>[2x]GTSTQTKAGSLTIVGTGIESIGQMTLQALSYIEAAAKVFYCVIDPATEAFILTKNKNCVDLYQYYDNGKSALNTYTQMSELMVREVRKGLDVVGVFYGHPGVFVNPSHRALAIAKSEGYRARMLPGVSAEDCLFADLCIDPSNPGCLTYEASDFLIRDRPVSIHSHLVLFQVGCVGIADFNFTGFDNNKFGVLVDRLEQEYGAEHPVVHYIAAMMPHQDPVTDKYTVAQLREPEIAKRVGGVSTFYIPPKARKASNLDIIRRLELLPAGQVPDKKARIYPANQWEPDVPEVEPYRPSDQAAIAQLADHAPPEQYQPLATSKAMSDVMTKLALDPKALADYKADHRAFAQSVPDLTPQERAALELGDSWAIRCAMKNMPSSLLDAARESGEEASQNGFPWVIVVGVIGVIG

While chemical methylation of an amide bond uses a strong base to generate the imidate, OphA, the precursor protein of the fungal peptide macrocycle omphalotin A, self-hypermethylates amides at pH 7 using S-adenosyl methionine (SAM) as cofactor. Omphalotin A derives from the C terminus of the OphA protein, and it is the OphA protein that methylates its own C terminus using S-adenosyl methionine (SAM). The structure of OphA reveals a complex catenane-like arrangement in which the peptide substrate is clamped with its amide nitrogen aligned for nucleophilic attack on the methyl group of SAM. Here, we report the structure of the peptide amide methyltransferase OphA including complexes with cofactor [SAM and S-adenosyl homocysteine (SAH)], cofactor analog, substrate, and product.

Y76F, R72A, R72K, and Y98A were unmethylated even after 3 days of overexpression in E. coli. In the R72A-SAM complex (rmsd of 0.7 Å over 720 Cα atoms with OphAΔC6-SAH), peptide bonds of the substrate residues i−1 and i are flipped 180° relative to the conformation observed in OphAΔC6 and Y63F-SAH. Although the side chain of residue i+1 sits in the same pocket as seen in the OphAΔC6 protein, its backbone has a different hydrogen bond arrangement. Consequently, the amide nitrogen at position i (Trp400) points away from SAM and is no longer aligned for methylation. The flipped peptide results in Arg72 adopting an alternative conformation. Despite the large conformational change in substrate peptide, conformations of other OphAΔC6 residues are essentially unaltered, pointing to rigidity at the active site. We therefore hypothesize that, by disrupting anchoring interactions, the flipped conformation can be adopted to relieve the steric clashes between SAM and the amide that would otherwise occur. We speculate that the flipped conformation of the substrate (seen in R72A, Y98A, and Y76F SAM complex structures) resembles an intermediate arrangement that occurs during translocation.> ISFKPGNQIDFNRLFTLPVTELFDPNTMFVYDQYVPLLVNLPSGFDQASIRLKVISYSVENQTLGVRLEFKDPQTQQFIPVLNASSTGPQTVFQPFNQ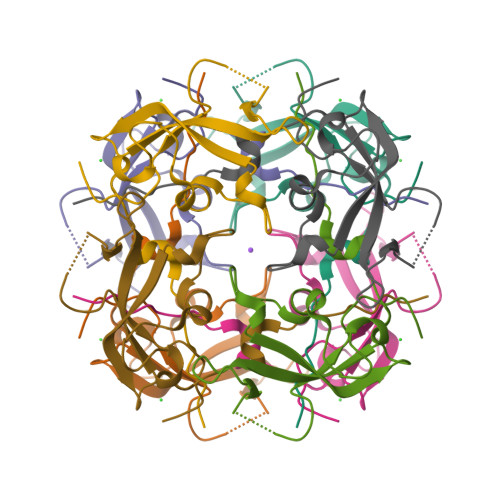WAD> MADVAGTSNRDFAGREQRLFNSEQYNYNNSLNGEVSVWVYAYYSDGSVLVINKNSQYKVGISETFKALKEYREGQHNDSYDEYEVNQSIYYPNGGDARKFHSNAKPRAIQIIFSPSVNVRTIKMAKGNAVSVPDEYLQRSHPWEATGIKYRKIKRDGEIVGYSHYFELPHEYNSISLAVSGVHKNPSSYNVGCCHNVMDVFQSCDLALRFCNRYWAELELVNHYISPNAYPYLDINNHSYGVALSN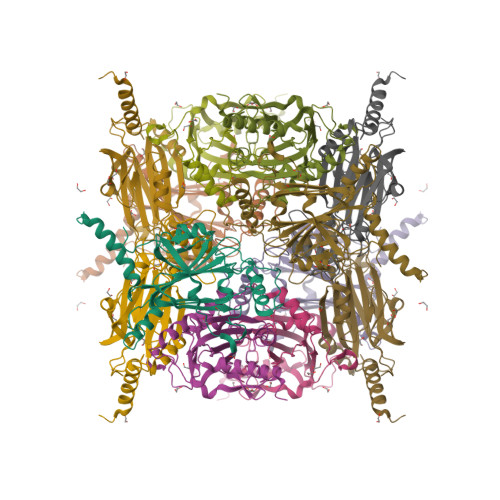RQ> IVGGKVCPKGECPWQVLLLVNGAQLCGGTLINTIWVVSAAHCFDKIKNWRNLIAVLGEHDLSEHDGDEQSRRVAQVIIPSTYVPGTTNHDIALLRLHQPVVLTDHVVPLCLPERTFSERTLAFVRFSLVSGWGQLLDRGATALELMVLNVPRLMTQDCL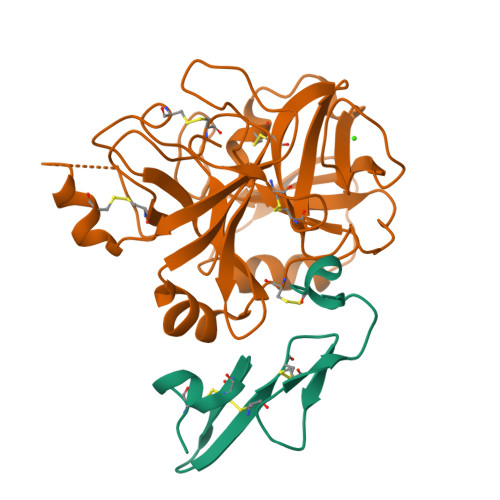QQSRKVGDSPNITEYMFCAGYSDGSKDSCKGDSGGPHATHYRGTWYLTGIVSWGQGCATVGHFGVYTRVSQYIEWLQKLMRSEPRPGVLLRAPFP;> HKDDQLICVNENGGCEQYCSDHTGTKRSCRCHEGYSLLADGVSCTPTVEYPCGKIPILEKRNASKPQGR>[2x]TGVTENTICKYGYLIQMSNHYECKCIEGYVLINEDTCGKKVVCDKVENSFKACDEYAYCFDLGNKNNEKQIKCMCRTEYTLTAGVCVPNVCRD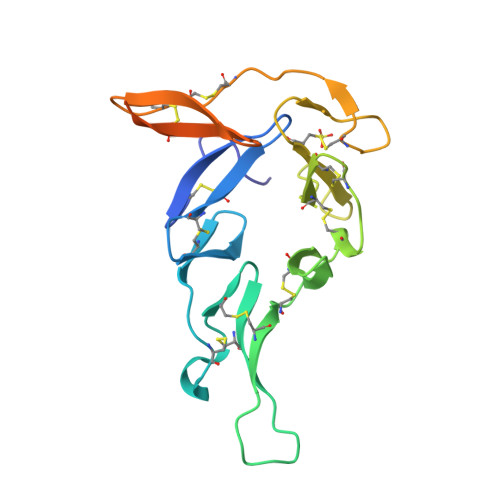KVCGKGKCIVDPANSLTHTCSCNIGTILNQNKLCDIQGDTPCSLKCAENEVCTLEGNYYTCKEDPSSNGGGNTVDQADTSYSGTKHHHHHH RgNanOx (RUMGNA_02695) from R. gnavus ATCC 29149 catalyzes the equilibration of 2,7-anhydro-Neu5Ac and Neu5Ac. The novel oxidoreductase identified in our work showed to catalyze the conversion 2,7-anhydro-Neu5Ac to Neu5Ac in the presence of NAD+ in a reversible manner. The protein shows a Rossman fold typical of NAD-binding protein of the Gfo/Idh/MocA class characterized by a central β-sheet with helices on either side. Here, we showed that RgNanOx acts through a multistep mechanism involving a keto intermediate and cycling of NADH/NAD+.

RgNanOx forms a dimer in the asymmetric unit, and the NAD+ cofactor can be seen bound to the protein. In the RgNanOx structure, there is additional density adjacent to the nicotinamide ring that, given the high resolution of the second structure, we were able to unambiguously identify as citric acid from the crystallization buffer. Oxidoreductase proteins typically have a catalytic triad of K (found in the EKP motif), D, and H (often found as a DXXXH motif; in some enzymes Y replaces the H) and a fourth residue, which is positively charged. RgNanOx has Lys-93 and His-178 which correspond to the Lys and His of the catalytic triad, and Lys-163 occupies the “fourth” position. However, RgNanOx has His-175, which occupies the position typical for the Asp in the catalytic triad. The closest structural match (0.8 Å over 341 residues) is the recently solved crystal structure of YjhC oxidoreductase from E. coli, which also has a HXXH motif. The following mutants of RgNanOx were constructed: K93A, K163A, H175A, H176A, and H178A. The purified mutants lost enzymatic activity, as demonstrated by electrospray ionization spray MS (ESI-MS), supporting the hypothesis that they are catalytically important.

> GAMKTVGYAIVGTGYFGAELGRIMKEQEGARIVAVLDPENGQTIAEELDCDVETDLDTLYSREDVEAVIVATPNYLHKEPVIKAAEHGVNVFCEKPIALSYQDCDEMVRTCQEHGVIFMAGHVMNFFHGVRYAKKLINDGVIGKVLYCHSARNGWEEQQPTISWKKIREKSGGHLYHHIHELDCVQFLMGGMPEEVTMTGGNVAHQGEAFGDEDDMLFVNMQFSDNRYAVLEWGSAFHWPEHYVLIQGTKGAIKIDMCDCGGTLKVDGREEHFLVHESQEEDDDRTRIYHGTEMDGAIMYGKPGKKPPMWLHSIMKNEMKYLNGILHGKEVDDEFRPLLTGEAARAAIATADACTKSRFEDRKVKLSEIIGEGS;> MKTVGYAIVGTGYFGAELGRIMKEQEGARIVAVLDPENGQTIAEELDCDVETDLDTLYSREDVEAVIVATPNYLHKEPVIKAAEHGVNVFCEKPIALSYQDCDEMVRTCQEHGVIFMAGHVMNFFHGVRYAKKLINDGVIGKVLYCHSARNGWEEQQPTISWKKIREKSGGHLYHHIHELDCVQFLMGGMPEEVTMTGGNVAHQGEAFGDEDDMLFVNMQFSDNRYAVLEWGSAFHWPEHYVLIQGTKGAIKIDMCDCGGTLKVDGREEHFLVHESQEEDDDRTRIYHGTEMDGAIMYGKPGKKPPMWLHSIMKNEMKYLNGILHGKEVDDEFRPLLTGEAARAAIATADACTKSRFEDRKVKLSEIIG>GPGSMSMADRDGKIWMDGKLIEWRDAKIHVLTHTLHYGMGVFEGVRAYKTADGGTAIFRLKEHTKRLLNSAKIFQMDVPFDQETLEAAQRDVVRENKLE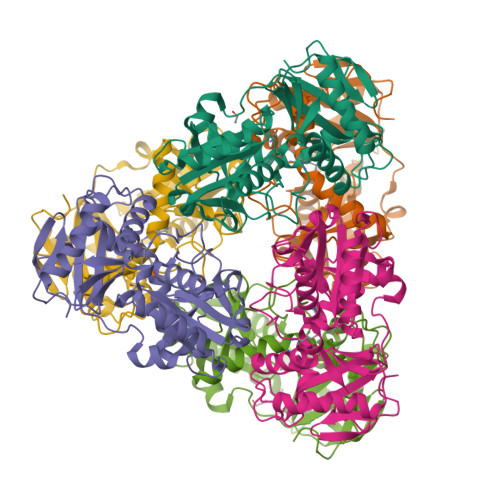SCYLRPIIWIGSEKLGVSAKGNTIHVAIAAWPWGAYLGEEGLAKGIRVKTSSFTRHHVNVSMVRAKASGWYVNSILANQEATADGYDEALLLDVDGYVSEGSGENFFLVNRGKLYTPDLASCLDGITRDTVITLAKEAGIEVIEKRITRDEVYTADEAFFTGTAAEVTPIRELDNRTIGGGARGPITEKLQSAFFDVVNGKSAKHADWLTKI[6x]> GHMQLLSRRLKLEKEVRNLQEQLITAETARKVEAKNEDKDLQTLIQKWKNAAQQAAEVLFKPMAERIRLAGGVTQSFRIEEGENKG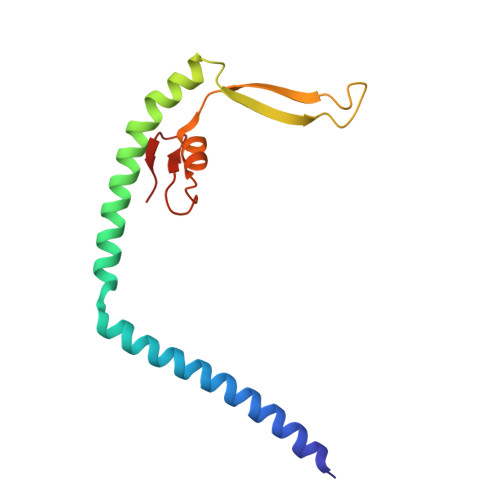QIQEVRTEFTMSMFLNQFGVPVHLMSFDEENGDWKS Several antibiotic resistance genes are found within the E. anophelis genome, including a chloramphenicol acetyltransferase (CAT). CATs play important roles in antibiotic resistance and can be transferred in genetic mobile elements. They catalyse the acetylation of the antibiotic chloramphenicol, thereby reducing its effectiveness as a viable drug for therapy. Homologs of this protein are important for bacterial Cm antibiotic resistance because they acetylate the 3′-hydroxyl group of Cm. Additionally, Type A CATs form a distinct structural group compared to Type B and C. All three types of proteins are trimers, but Type B and C adopt a hexapeptide repeat structural fold, which is not found in Type A.

Here, we determined the high-resolution crystal structure of a CAT protein from the E. anophelis NUHP1 strain that caused a Singaporean outbreak. The electron density map allowed all residues of the protein (1-208) to be modeled. A single protein monomer was present in the asymmetric unit of the crystal with the topology shown in Fig. 2A. The monomer contained two main domains: (1) a left-handed β-helix core (15 β-strands spanning residues 12-163) forms a prism at the center of the monomer and contains two extended loop regions (44-56 and 72-110), and (2) a C-terminal α-helical domain comprised of three α-helices (spanning residues 164-208). The only biological assembly predicted from PISA for the E. anophelis CAT enzyme was a trimer, which is identical to all other structurally characterized CAT enzymes. In our E. anophelis CAT structure, we found one interface mediating the trimer formation. In total, the interface forms 21 hydrogen bonds, two salt bridges, and buries 1699.8 Å2 of solvent accessible surface area (ASA). Therefore, the results of the sequence and structural comparisons indicate the E. anophelis protein is most likely a Type B CAT. The residues that could potentially hydrogen bond with Cm in the binding site of the E. anophelis structure include Pro8, Gly11, Tyr30, and Ser32 from one monomer and His79 from a second monomer. These residues are all identical in the CAT enzyme from P. aeruginosa (PDB ID: 2XAT29).

> MAHHHHHHMKNFFESPFKGKIIKDHIQNPNIIAGKYSYYSGYYHGHSFDDCARYLLPDRNDVDKLIIGSYCSVGTGASFIMAGNQGHRYDWISSFPFFYMNEVEAFENSIDAFKNAGDTIIGNDVWIGGEAMIMPGIKIGDGAVIGSRALVTKDVEPYAIVGGNPAKLIKKRFSENQIAILLEIKWWEWNEEVLADAMPILCSGNIDLLYKFYKNI> 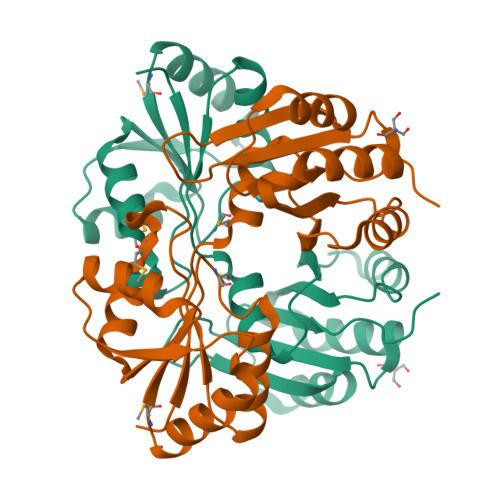QGHMEQQRSFQTETGGHLYLVPTPIGNLDDMTFRAVKTLTAVDLIAAEDTRNTQKLLNHFEITTKQISFHEHNTQERIPQLIAKLKQGMQIAQVSDAGMPSISDPGHELVNACIDAHIPVVPLPGANAGLTALIASGLAPQPFYFYGFLDRKPKDRKAEIAGLAQRPETLIFYEAPHRLKKTLQNLAAGFGDERPAVLCRELTKRYEEFLRGSLAELANWAATDTVRGEFVVLVGGNPAPTTAATTAVDLSEPIDVQVDRLIAAGEKPNDAIKEVAKLRGAKKQEIYRQYHHLDEE>[2x]GSHMAVELNHTIVLVKDKDASATFMADLLGLPKPKEMGPFAVLQLANDVSIDFMDFRGEGDIVPGHCAFLISDEEFDQIFGRIREGGIEH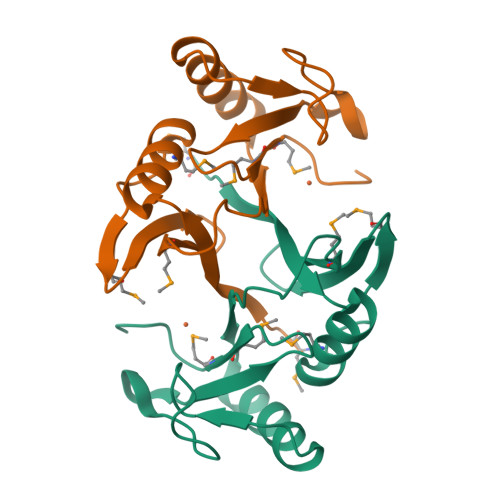WADQYHREPGRINDRDGGRGVYFEDPSGHNMEIMTRPYGSGGA>MKRVSRRAFLRRLGVGVAATAAFSPLAVAQARRYRWRIQTAWDAGTVGYSLFQKFTERVKELTDGQLEVQPFPAGAVVGTFDMFDAVKTGVLDGMNPFTLYWAGRMPVTAFLSSYALGLDRPDQWETWFYSLGGLDIARRAFAEQGLFYVGPVQHDLNIIHSKKPIRRFEDFKGVKLRVPGGMIAEVFAAAGASTVLLPGGEVYPALERGVIDAADFVGPAVNYNLGFHQVAKYIIMGPPETPAIHQPVDLMDFTINLNRWRSLP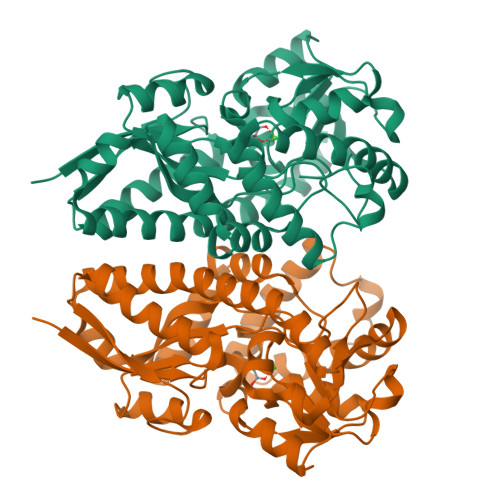KPLQERFIAAVHEYSWIHYAGIQKANLEAWPKYRQAGVEVIRLSNEDVRKFRRLAIPIWFKWAKMDKYSREAFASQLEYMKGIGYVTDEELKGLSL[2x]> KKKRLTKADIGTPSNFQHIGHVGWDPNTGFDLNNLDPELKNLFDMCGISEAQLKDRETSKVIYDFIEKTGGVEAVKNELRRQAENLYFQGLEH;> MGKKSPDSSQGASGPAMQSPSGPTIRPTRPAPPPPTTGGANAKRPATHGKGRAPQPPTAGSSSGSEQPTAMSSEVAKLVSELKDAVHSHAESQKVLKKVSQELQTKWTDWENNRGPDYLLHGYRVIARALQQTYTEQSMLIEGTSSTGPVPQAVTVAKDAVTQTVRGAIKNLENPKPGNDPDGVLMQVVISLGIEGPTLDPGESIQNFLETRVSDFGGDDSDIDYTSDIARLGSALDRVRENHPNEMPRIWIALARELGAAVHSHATSVRIANAGKNHTRDVVRMANESSRLLQGMKVLSVGAWANTMTVLIGDLFEHHHHHHHHH

To enter epithelial cells, the obligate intracellular pathogen Chlamydia pneumoniae secretes early effector proteins, which bind to and modulate the host-cell’s plasma membrane and recruit several pivotal endocytic host proteins. The early secreted Cpn effector protein SemD binds to the inner leaflet of the PM below the invading EB and directly recruits G-actin and the essential endocytic proteins SNX9 and N-WASP12. During a Cpn infection, the C-terminus of the membrane-bound SemD interacts with the BR-GBD domain of N-WASP, thus triggering N-WASP activation and Arp2/3-mediated actin polymerisation via an unknown mechanism. We demonstrate that SemD, a protein of 382 aa, can interact simultaneously with the PM, SNX9 and N-WASP, thereby combining membrane association and deformation with modulation of the actin polymerisation machinery.

To understand the activation of N-WASP by SemD, we structurally analysed the complex formed by recombinant SemDΔAPH and the BR-GBD domain of N-WASP. The co-crystal of SemDΔAPH in complex with BR-GBD yielded a structure with a medium resolution of 3.3 Å, which is attributable to the flexible termini of both proteins. Interestingly, the loop connecting helices 2 and 3 (208-GTSSTG−213) of SemDΔAPH is stabilised in the complex and can now be modelled. Despite the moderate resolution of the crystals containing the SemDΔAPH – BR-GBD complex, the interaction surface between the two proteins is well resolved. Comparison of the structures of SemDΔAPH alone and in complex with BR-GBD revealed virtually identical conformations of the SemD core regions, as indicated by a low RMSD of 0.7 Å. We found three positively charged residues within the BR domain of N-WASP (K193, R194 and K197) that interact directly with the negatively charged area found on the front of SemD, formed by helices α1, α2, α5 and α9. Additionally, five residues of the N-WASP CRIB domain engage with residues in the SemD binding groove, mainly formed by helix α4, the adjacent loop and helix α9. The N-WASP C-sub domain is located underneath the helical arrangement of SemDΔAPH, flanked by its extended helix α1. Owing to the flexibility of the N-terminal domains of SemDΔAPH and BR-GBD, these regions are not resolved in the crystal structure of the complex. Our structural and biochemical data further reveal that SemD provides the negatively charged patch and the binding groove required for selective binding of the positively charged C-terminal part of the BR and the CRIB domains of N-WASP, respectively, thus mimicking Cdc42GTP-mediated N-WASP activation.>[2x]GSHMAFKKPLSVFKGPLLHISPAEELYFGSTESGEKKTLIVLTNVTKNIV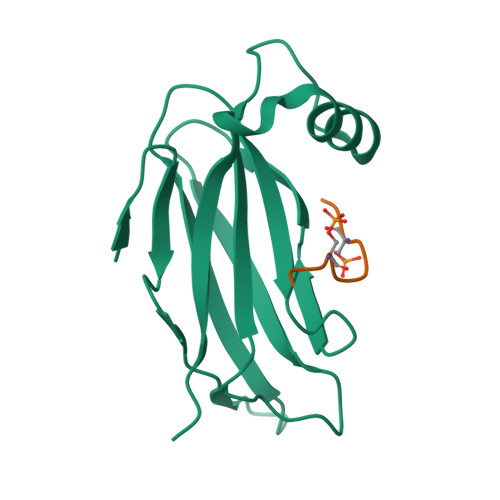AFKVRTTAPEKYRVKPSNSSCDPGASVDIVVSPHGGLTVSAQDRFLIMAAEMEQSSGTGPAELTQFWKEVPRNKVMEHRLRCHTV;>[2x]CLFSGALSEGQFYSPPESFAG> MKTEWPELVGKSVEEAKKVILQDKPAAQIIV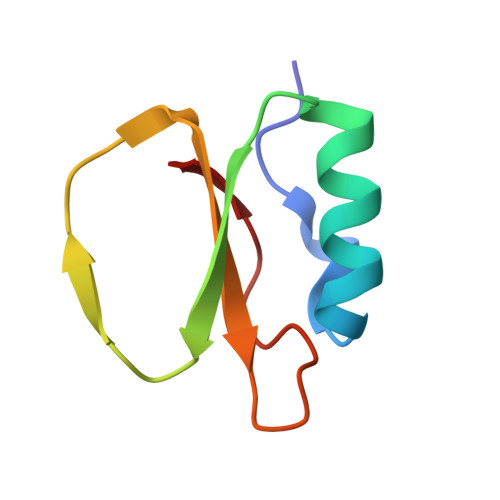LPVGTIVTMAYRIDRVRLFVDRLDNIAQVPRVG> MDVSFRLSGATSSSYGVFISNLRKALPNERKLYDIPLLRSSLPGSQRYALIHLTNYADETISV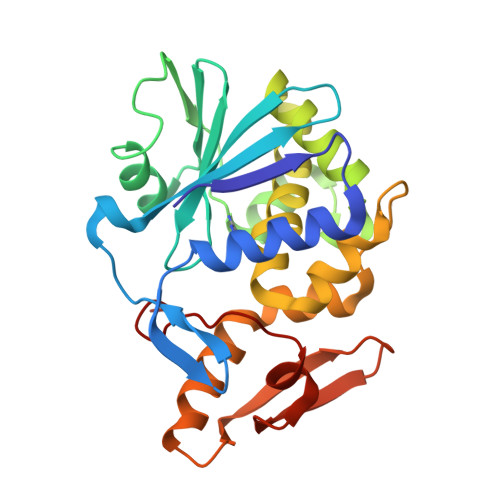AIDVTNVYIMGYRAGDTSYFFNEASATEAAKYVFKDAMRKVTLPYSGNYERLQTAAGKIRENIPLGLPALDSAITTLFYYNANSAASALMVLIQSTSAAARYKFIEQQIGKRVDKTFLPSLAIISLANSWSALSKQIQIASTNNGQFESPVVLINAQNQRVTITNVDAGVVTSNIALLLNRNNMA> EGPTFQDVASQVFGQPVGPDNDGTLYIFGLTAKYTEPEYVDGRGPYKSFLKMLPSIRWYDPEHYWTNGSQTEGVFKNEECVLCHTVQTPTIVNDWKQSSHGSKDIRRGIGIKKDGKPVEDLVGCADCHGNNHQKLEMPTYKLCNDCHPKETAEHRAGGLGSHTHAYTVNVLEFSWHVGKPAEEVTGCAHCHAIAENRC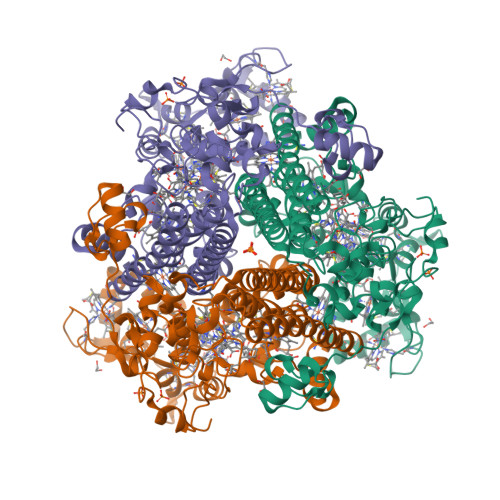SGCHTRHKFDPAEARKPTACRVCHMGIDHDEWAMYNTSIHGALYEAESARMDWGKKLKKGNYRVPTCAYCHMQNGDHNPQRFGTIYSDMGMFQVDRGAPKHKAKRDSWIKLCQDCHSPRFAADKLKEMDAGVNLSFTKWREAAAVIVGCYLDGVVDPMPEGSAPDWYGHYTFSLLPGGDPRFYATSNLERLGLEMICYLTGNVYKAYAHMSMYNQTYGNGSAFEQDRKLVEIKTEAAKLRRFAAIEKKIGLEHKSADFWKHGEYLDLLPGWKRKPGDVDVEWFKRTDIPHRANADAGVEIHH> XXXXXXXXXXXXXXXXXXXXXXXXXXXXXXXXXXXXXXXXXXXXXXXXXXXXXXXXXXXXXXXXXXXXXXXXXXXXXXXXXXXXXXXXXXXXXXXXXXXXXXXXXXXXXXXXXXXXXXXXXXXXXXXXXXXXXXXXXXXXXXXXXXXXXXXXXXXXXXXXXXXXXXXXXXXXXXXXXXXXXXXXXXXXXXXXXXXXXXXXXXXXXXXXXXXXXXXXXXXXXXXXXXXXXXXXXXXXXXXXXXXXXXXXXXXXXXXXXXXXXXXXXXXXXXXXXXXXXXXXXXXXXXXXXXXXXXXXXXXXXXXXXXFSTNFRDTVDILVGWHIDHTQKPSLTQQVSGWLQSLEPFWVADLAFSTTLLGQFLEDMEAYAEDLSHVASGESVDEDVPPPSVSLPKLAALLRVFSTVVRSIGERFSPIRGPPITEAYVTDVLYRVMRCVTAANQVFFSEAVLTAANECVGVLLGSLDPSMTIHCDMVITYGLDQLENCQTCGTDYIISVLNLLTLIVEQINTKLPSSFVEKLFIPSSKLLFLRYHKEKEVVAVAHAVYQAVLSLKNIPVLETAYKLILGEMTCALNNLLHSLQLPEACSEIKHEAFKNHVFNVDNAKFVVIFDLSALTTIGNAKNSLIGMWALSPTVFALLSKNLMIVHSDLAVHFPAIQYAVLYTLYSHCTRHDHFISSSLSSSSPSLFDGAVISTVTTATKKHFSIILNLLGILLKKDNLNQDTRKLLMTWALEAAVLMRKSETYAPLFSLPSFHKFCKGLLANTLVEDVNICLQACSSLHALSSSLPDDLLQRCVDVCRVQLVHSGTRIRQAFGKLLKSIPLDVVLSNNNHTEIQEISLALRSHMSKAPSNTFHPQDFSDVISFILYGNSHRTGKDNWLERLFYSCQRLDKRDQSTIPRNLLKTDAVLWQWAIWEAAQFTVLSKLRTPLGRAQDTFQTIEGIIRSLAAHTLNPDQDVSQWTTADNDEGHGNNQLRLVLLLQYLENLEKLMYNAYEGCANALTSPPKVIRTFFYTNRQTCQDWLTRIRLSIMRVGLLAGQPAVTVRHGFDLLTEMKTTSLSQGNELEVTIMMVVEALCELHCPEAIQGIAVWSSSIVGKNLLWINSVAQQAEGRFEKASVEYQEHLCAMTGVDCCISSFDKSVLTLANAGRNSASPKHSLNGESRKTVLSKPTDSSPEVINYLGNKACECYISIADWAAVQEWQNSIHDLKKSTSSTSLNLKADFNYIKSLSSFESGKFVECTEQLELLPGENINLLAGGSKEKIDMKKLLPNMLSPDPRELQKSIEVQLLRSSVCLATALNPIEQDQKWQSITENVVKYLKQTSRIAIGPLRLSTLTVSQSLPVLSTLQLYCSSALENTVSNRLSTEDCLIPLFSEALRSCKQHDVRPWMQALRYTMYQNQLLE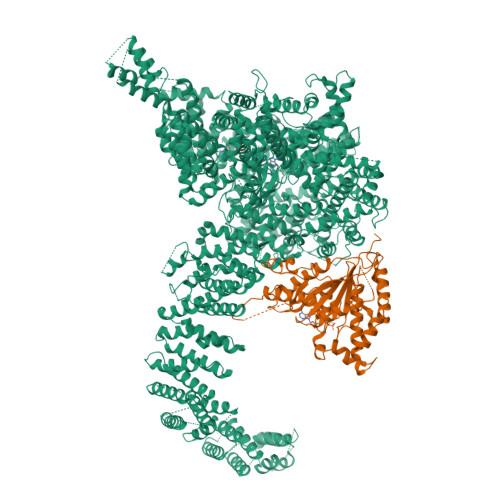KIKEQTVPIRSHLMELGLTAAKFARKRGNVSLATRLLAQCSEVQLGKTTTAQDLVQHFKKLSTQGQVDEKWGPELDIEKTKLLYTAGQSTHAMEMLSSCAISFCKSVKAEYAVAKSILTLAKWIQAEWKEISGQLKQVYRAQHQQNFTGLSTLSKNILTLIELPSVNTMEEEYPRIESESTVHIGVGEPDFILGQLYHLSSVQAPEVAKSWAALASWAYRWGRKVVDNASXXXXXXXXXXXXXXXXXXXXXXXXXXXXXXXXXXXXXXXXXXXXXXXXXXXXXXXXXXXXXXXXXXXXXXXXXXXXXXXXXXXXXXXXEGVIKVWRKVVDRIFSLYKLSCSAYFTFLKLNAGQIPLDEDDPRLHLSHRVEQSTDDMIVMATLRLLRLLVKHAGELRQYLEHGLETTPTAPWRGIIPQLFSRLNHPEVYVRQSICNLLCRVAQDSPHLILYPAIVGTISLSSESQASGNKFSTAIPTLLGNIQGEELLVSECEGGSPPASQDSNKDEPKSGLNEDQAMMQDCYSKIVDKLSSANPTMVLQVQMLVAELRRVTVLWDELWLGVLLQQHMYVLXXXXXXXXXXXXXXXXXXXXXXXXXXXXXXXXXXXXXXXXXXXXXXXXXXXXXXXXPHEKWFQDNYGDAIENALEKLKXXXXXXXXXXXXXXXXXXXXXXXXXXXXXXXYILRLEEISPWLAAMTNTEIALPGEVSARDTVTIHSVGGTITILPTKTKPKKLLFLGSDGKSYPYLFKGLEDLHLDERIMQFLSIVNTMFATINRQETPRFHARHYSVTPLGTRSGLIQWVDGATPLFGLYKRWQQREAALQAQKAQDSYQTPQNPGIVPRPSELYYSKIGPALKTVGLSLDVSRRDWPLHVMKAVLEELMEATPPNLLAKELWSSCTTPDEWWRVTQSYARSTAVMSMVGYIIGLGDRHLDNVLIDMTTGEVVHIDYNVCFEKGKSLRVPEKVPFRMTQNIETALGVTGVEGVFRLSCEQVLHIMRRGRETLLTLLEAFVYDPLVDWTAGGEAGFAGAVYGGGGQQAESKQSKREMEREITRSLFSSRVAEIKVNWFKNRDEMLVVLPKLDGSLDEYLSLQEQLTDVEKLQGKLLEEIEFLEGAEGVDHPSHTLQHRYSEHTQLQTQQRAVQEAIQVKLNEFEQWITHYQAAFNNLEATQLASLLQEISTQMDLGPPSYVPATAFLQNAGQAHLISQCEQLEGEVGALLQQRRSVLRGCLEQLHHYATVALQYPKAIFQKHRIEQWKTWMEELICNTTVERCQELYRKYEMQYAPQPPPTVCQFITATEMTLQRYAADINSRLIRQVERLKQEAVTVPVCEDQLKEIERCIKVFLHENGEEGSLSLASVIISALCTLTRRNLMMEGAASSAGEQLVDLTSRDGAWFLEELCSMSGNVTCLVQLLKQCHLVPQDLDIPNPMEASETVHLANGVYTSLQELNSNFRQIIFPEALRCLMKGEYTLESMLHELDGLIEQTTDGVPLQTLVESLQAYLRNAAMGLEEETHAHYIDVARLLHAQYGELIQPRNGSVDETPKMSAGQMLLVAFDGMFAQVETAFSLLVEKLNKMEIPIAWRKIDIIREARSTQVNFFDDDNHRQVLEEIFFLKRLQTIKEFFRLCGTFSKTLSGSSSLEDQNTVNGPVQIVNVKTLFRNSCFSEDQMAKPIKAFTADFVRQLLIGLPNQALGLTLCSFISALGVDIIAQVEAKDFGAESKVSVDDLCKKAVEHNIQIGKFSQLVMNRATVLASSYDTAWKKHDLVRRLETSISSCKTSLQRVQLHIAMFQWQHEDLLINRPQAMSVTPPPRSAILTSMKKKLHTLSQIETSIATVQEKLAALESSIEQRLKWAGGANPALAPVLQDFEATIAERRNLVLKESQRASQVTFLCSNIIHFESLRTRTAEALNLDAALFELIKRCQQMCSFASQFNSSVSELELRLLQRVDTGLEHPIGSSEWLLSAHKQLTQDMSTQRAIQTEKEQQIETVCETIQNLVDNIKTVLTGHNRQLGDVKHLLKAMAKDEEAALADGEDVPYENSVRQFLGEYKSWQDNIQTVLFTLVQAMGQVRSQEHVEMLQEITPTLKELKTQSQSIYNNLVSFASPLVTDATNECSSPTSSATYQPSFAAAVRSNTGQKTQPDVMSQNARKLIQKNLATSADTPPSTVPGTGKSVACSPKKAVRDPKTGKAVQERNSYAVSVWKRVKAKLEGRDVDPNRRMSVAEQVDYVIKEATNLDNLAQLYEGWTAWV;> AKLLPPERMKHSIKLVDDQMNWCDSAIEYLLDQTDVLVVGVLGLQGTGKSMVMSLLSANTPEEDQRTYVFRAQSAEMKERGGNQTSGIDFFITQERIVFLDTQPILSPSILDHLINNDRKLPPEYNLPHTYVEMQSLQIAAFLFTVCHVVIVVQDWFTDLSLYRFLQTAEMVKPSTPSPSHESSSSSGSDEGTEYYPHLVFLQNKARREDFCPRKLRQMHLMIDQLMAHSHLRYKGTLSMLQCNVFPGLPPDFLDSEVNLFLVPFMDSEAESENPPRAGPGSSPLFSLLPGYRGHPSFQSLVSKLRSQVMSMARPQLSHTILTEKNWFHYAARIWDGVRKSSALAEYSRLLA1-DEOXYMANNOJIRIMYCIN | C6 H13 N O4 | 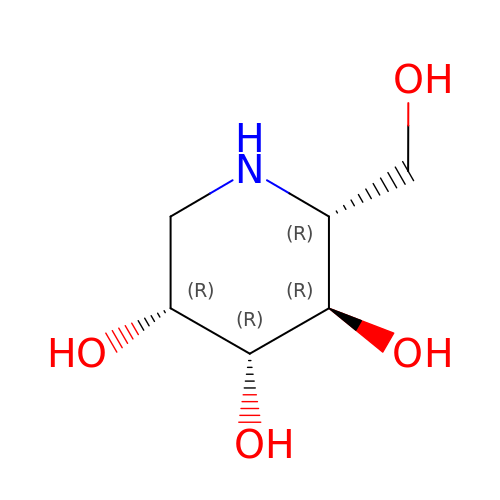LXBIFEVIBLOUGU-KVTDHHQDSA-N The NanH sialidase of Tannerella forsythia, one of the bacteria associated with severe periodontal disease plays a role in virulence. The C-terminal catalytic domain is preceded by a 160 amino acid N-terminal domain that is a CBM that our laboratory discovered is capable of binding various sialoglycans and non-sialylated derivatives but has no catalytic activity itself. The NanH catalytic domain (residues 197–552) folds into a characteristic 6-bladed β-propeller catalytic domain, with each blade being composed of 3–4 antiparallel β-strands.

After establishing the IC50 of these inhibitors with purified NanH, we attempted co-crystallisation and crystal soaking with DANA and Oseltamivir since both had IC50 in the μM range. While we were unable to identify DANA in any crystal models, we could solve a model at 1.9 Å with Oseltamivir in the active site after soaking it into the NanH-apo crystals at a concentration of 5 mM. The electron density for the oseltamivir is notably poorer in one subunit and could not be modelled reliably, implying a lower occupancy of the site, although the reason for this is not clear as access appears equivalent and the local protein residues adopt the same conformations. In this model, Oseltamivir is orientated in the active site via its negatively charged carboxyl group, which is held equatorial to the cyclohexene ring through hydrogen bonding interactions with the guanidiniums of the arginine triad. The cyclohexene ring itself is sitting in a distorted boat conformation caused by the carboxyl group taking a pseudoequatorial position upon the binding of the arginine triad. The amino group of oseltamivir (position C9) interacts with the carboxylates of D237 and D280 while the N-acetyl tail sits in a hydrophobic pocket with a hydrogen bond forming between the amide of the N-acetyl and the carboxylate of D280. Comparison of the active site conformation between the NanH-apo and oseltamivir bound form shows that all residues have identical conformations except for the sidechain of W308 which is displaced by the pentyl ether group of oseltamivir, with an average displacement for the aromatic rings of the tryptophan of 1.4 Å. There are no other major differences in the structure of the protein backbone or sidechains compared with NanH-apo. The oseltamivir-dependent distortion may be attributed to its competitive inhibitory mechanism where it binds into the active site, but also suggests this region may be a target for the introduction of further modifications of oseltamivir in the design of a new inhibitor molecule.

>[2x]DSVYVQNPQIPILVDRTDNVLFRIRIPDATKGDVLNRLTIRFGNEDKLSEVKAVRLFYAGTEAATKGRSRFAPVTYVSSHNIRNTRSANPSYSIRQDEVTTVANTLTLKTRQPMVKGINYFWVSVEMDRNTSLLSKLTSTVTEVVINDKPAVIAGEQAAVRRMGIGVRHAGDDGSASFRIPGLVTTNKGTLLGVYDVRYNNSVDLQEHIDVGLSRSTDKGQTWEPMRIAMSFGETDGLPSGQNGVGDPSILVDERTNTVWVVAAWTHGMGNARAWTNSMPGMTPDETAQLMMVKSTDDGRTWSESTNITSQVKDPSWCFLLQGPGRGITMRDGTLVFPIQFIDSLRVPHAGIMYSKDRGETWHIHQPARTNTTEAQVAEVEPGVLMLNMRDNRGGSRAVSITRDLGKSWTEHSSNRSALPESICMASLISVKAKDNIIGKDLLLFSNPNTTEGRHHITIKASLDGGVTWLPAHQVLLDEEDGWGYSCLSMIDRETVGIFYESSVAHMTFQAVKIKDLIR> SMPEITGQVSLPPGKRTNLRKTGSERIAHGMRVKFNPLALLLDSSLEGEFDLVQRIIYEVDDPSLPNDEGITALHNAVCAGHT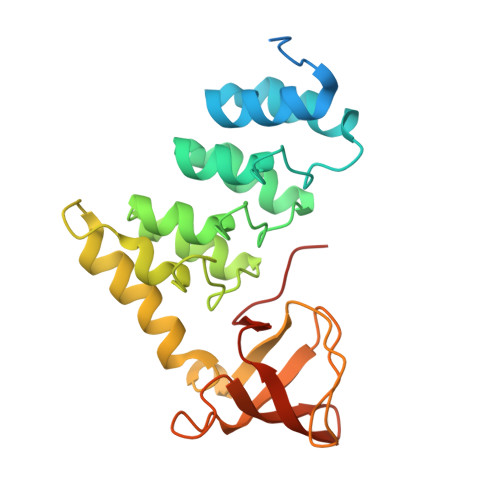EIVKFLVQFGVNVNAADSDGWTPLHCAASCNNVQVCKFLVESGAAVFAMTYSDMQTAADKCEEMEEGYTQCSQFLYGVQEKMGIMNKGVIYALWDYEPQNDDELPMKEGDCMTIIHREDEDEIEWWWARLNDKEGYVPRNLLGLYPRIKPRQRSLA>[4x]MNGVAAALLVWILTSPSSSDHGSENGWPKHTACNSGGLEVVYQSCDPLQDFGLSIDQCSKQIQSNLNIRFGIILRQDIRKLFLDITLMAKGSSILNYSYPLCEEDQPKFS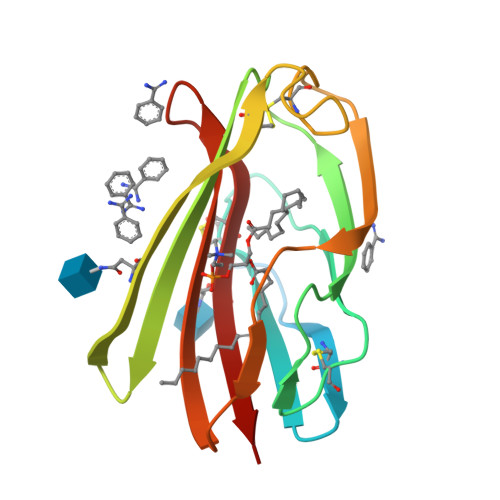FCGRRKGEQIYYAGPVNNPGLDVPQGEYQLLLELYNENRATVACANATVTSS Acetate kinase catalyzes reversible transfer of a γ-phosphate from ATP to acetate in the presence of a divalent metal ion. In the present study, we report the biochemical characterization and structures of S. typhimurium AckA (StAckA, NCBI accession: NP_461279.1, residues: 400, molecular mass: 43.3 kDa) in two crystal forms at 2.70 Å (apo, Form-I) and 1.90 Å (citrate-bound, Form-II) resolutions. StAckA protomer consists of two domains with characteristic βββαβαβα topology of ASKHA superfamily of proteins. A cleft between the two domains forms the active site pocket of StAckA.

Another crystal form of StAckA (Form-II) was obtained in the presence of citrate. The structure of this form was determined at 1.90 Å resolution using a polyalanine model of the Form-I StAckA monomer. Although the overall polypeptide fold in these two forms is similar, residues 230–300 (variable segment) were in significantly different conformations in the two subunits of Form-II dimer and these conformations in turn were different from that observed for this segment in Form-I. Residues 277–287 of B-subunit are close to the active site cleft present between the domains and occupy the space where ligands are expected to bind. B-subunit of Form-II represents the most closed state while A-subunit represents a conformation between those of Form-I and B-subunit of Form-II (data not shown). As the residues of the variable segment are also involved in the formation of active site pocket, Form-II structure is not suitable for binding nucleotides and therefore may represent an inhibited state of the enzyme. Examination of the difference electron density map of Form-II StAckA showed significant uninterpreted density located at the dimeric interface that was distinct from that of the polypeptide chain. Citrate, a component of the crystallization condition, was found to best fit the density and could be refined with reasonable B-factors (33.9 Å2) and occupancy (0.75). Interestingly, only one citrate binds at the dimeric interface resulting in an asymmetric dimer. It interacts with atoms (distance cutoff: ≤5.0 Å) of residues Arg178, Asp227, Thr228, Ser229, Met230, Asp257, Thr258, Leu259, Gly260, Arg309, Lys312 and Tyr313 of the A-subunit and Arg309, Lys312 and Tyr313 of the B-subunit.

>MRGSHHHHHHGMASHMSSKLVLVLNCGSSSLKFAIIDAVNGDEYLSGLAECFHLPEARIKWKMDGSKQEAALGAGAAHSEALNFIVNTILAQKPELSAQLTAIGHRIVHGGEKYTSSVVIDESVIQGIKDSASFAPLHNPAHLIGIAEALKSFPQLKDKNVAVFDTAFHQTMPEESYLYALPYSLYKEHGVRRYGAHGTSHFYVTQEAAKMLNKPVEELNIITCHLGNGGSVSAIRNGKCVDTSMGLTPLEGLVMGTRSGDIDPAIIFHLHDTLGMSVDQINKMLTKESGLLGLTEVTSDCRYVEDNYATKEDAKRAMDVYCHRLAKYIGSYTALMDGRLDAVVFTGGIGENAAMVRELSLGKLGVLGFEVDHERNLAARFGKSGFINKEGTRPAVVIPTNEELVIAQDASRLTA[2x]13-methyl-13,14-dihydro[1,3]benzodioxolo[5,6-c][1,3]dioxolo[4,5-i]phenanthridine | C20 H15 N O4 | 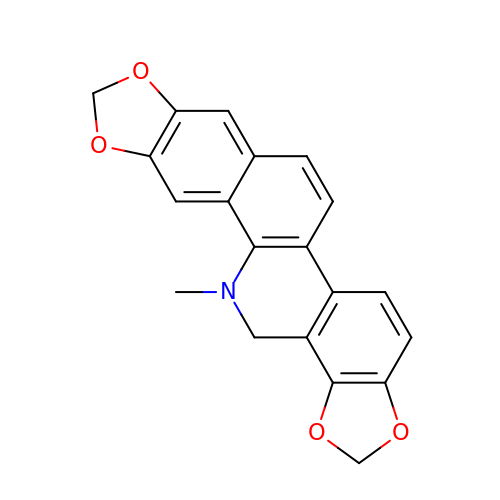CIUHLXZTZWTVFL-UHFFFAOYSA-N>MGSSHHHHHHSSGRENLYFQGHMPEVIFNGPAGRLEGRYQPSKEKSAPIAIILHPHPQFGGTMNNQIVYQLFYLFQKRGFTTLRFNFRSIGRSQGEFDHGAGELSDAASALDWVQSLHPDSKSCWVAGYSFGAWIGMQLLMRRPEIEGFMSIAPQPNTYDFSFLAPC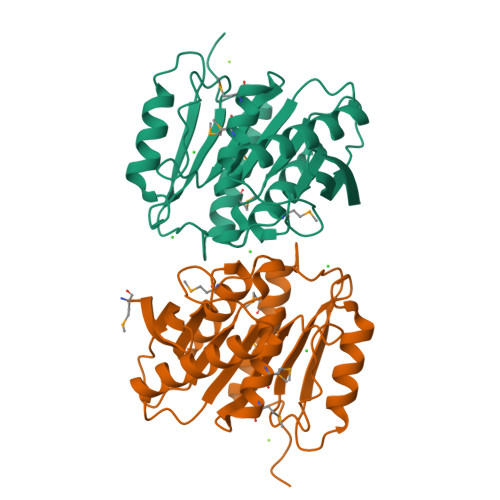PSSGLIINGDADKVAPEKDVNGLVEKLKTQKGILITHRTLPGANHFFNGKVDELMGECEDYLDRRLNGELVPEPAAKRIRGS[2x]>[2x]SLSPSARRVQGALETRGFGHLKVVELPASTRTAKEAAQAVGAEVGQIVKSLAYGGSKGAYLFLVSGKNRLDLGKAARLVGTDLLELDKWAVAALTGFAAGGVPPVG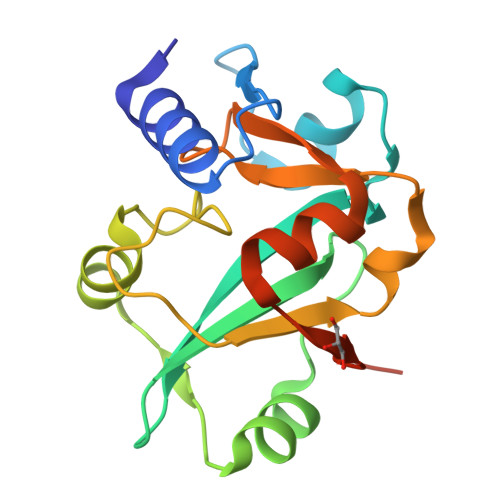HNTPLPAYLDEDLLGYPEVWAAGGTPRALFRATPKELLALTGAQVADLKEGLEHHHHHH> FISRFAPDQPRKGADILVEALERQGVETVFAYPGGASMEIHQALTRSSSIRNVLPRHEQGGVFAAEGYARSSGKPGICIATSGPGATNLVSGLADALLDSVPLVAITGQVPRRMIGTDAFQETPIVEVTRSITKHNYLVMDVEDIPRIIEEAFFLATSGRPGPVLVDVPKDIQQQLAIPNWEQAMRLPGYMSRMPKPPEDSHLEQIVRLISESKKPVLYVGGGCLNSSDELGRFVELTGIPVATTLMGLGSYPCDDELSLHMLGMHGTVYANYAVEHSDLLLAFGVRFDDRVTGKLEAFASRAKIVHIDIDSAEIGKNKTPHVSVCGDVKLALQGMNKVLENRAEELKLDFGVWRNELNVQKQKFPLSFKTFGEAIPPQYAIKVLDELTDGKAIISTGVGQHQMWAAQFYNYKKPRQWLSSGGLGAMGFGLPAAIGASVANPDAIVVDIDGDGSFIMNVQELATIRVENL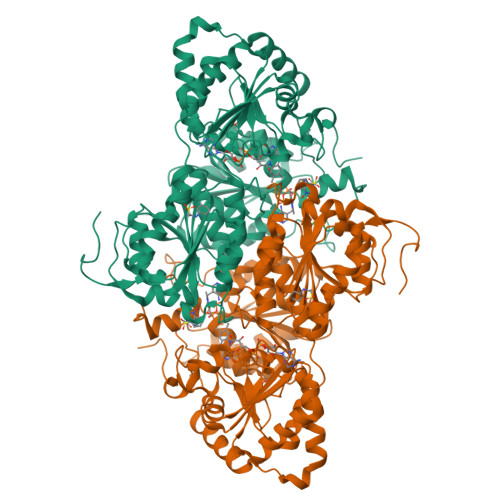PVKVLLLNNQHLGMVMQWEDRFYKANRAHTFLGDPAQEDEIFPNMLLFAAACGIPAARVTKKADLREAIQTMLDTPGPYLLDVICPHQEHVLPMIPSGGTFNDVITEGDGRIKY>GVQLTAAQELMIQQLVAAQLQCNKRSFSDQPKVTPWPLGADPQSRDARQQRFAHFTELAIISVQEIVDFAKQVPGFLQLGREDQIALLKASTIEIMLLETARRYNHETECITFLKDFTYSKDDFHRAGLQVEFINPIFEFSRAMRRLGLDDAEYALLIAINIFSADRPNVQEPGRVEALQQPYVEALLSYTRIKRPQDQLRFPRMLMKLVSLRTLSSVHSEQVFALRLQDKKLPPLLSEIWDVHE[3x]

The liver X receptors (LXRs) alpha (LXRα, NR1H3) and beta (LXRβ, NR1H2) are members of the nuclear hormone receptor (NHR) superfamily of transcription factors that function as heterodimers with the retinoid X receptor (RXR) and activate or repress gene expression in response to binding of cholesterol derivatives or synthetic ligands. Transcriptional responses of LXRs are known to directly result from ligand-induced conformational changes in the receptor: similarly to other NHRs, in the absence of ligands or in the presence of antagonists, LXRs form complexes with corepressors, while binding of agonist ligands forces the C-terminal helix H12 of the receptor to fold into the active state that creates an activation function-2 (AF-2) coactivator-binding surface. Reaching isoform selectivity by rational structure-based drug design has proven to be difficult since the ligand-binding pockets (LBPs) of LXRα and LXRβ are virtually identical. Since the adverse lipogenic effects are considered to be largely driven by LXRα23,28, drug discovery efforts have focused on developing LXRβ-selective compounds.

In this study, we compared AZ876 with structurally related compounds AZ1–6. These compounds have a central cyclic sulfone amide scaffold with lipophilic substituents on both sides identical to AZ876, except for the tert-butyl substituent replaced by a propyl group in AZ1–3 and AZ6. The third substituent from the core is a larger elongated amine linker that is different in AZ1–6. The amine linker is mostly lipophilic with a polar group at the far end. The compounds AZ1, AZ3, and BMS-852927 have the highest affinities of 2, 4, and 3 nM, and the compounds AZ6, AZ7, and 24,25EC have the lowest affinities of 161, 105, and 133 nM, respectively. Analysis of crystal structures of LXRβ LBD in complex with WAY-254011, AZ3, AZ6, and AZ8, as well as of previously published crystal structures of LXRβ31,40,55 reveals that GW3965 and BMS-852927 are the only compounds not forming a direct hydrogen bond with LXRβ His435 and therefore they do not stabilize the His435–Trp457 activation switch crucial for the agonistic conformation of H12. Other agonists form shorter hydrogen bonds of 2.5–3.1 Å essential for proper position of H12, which correlates with their activities both in LXRβ HDX-MS and functional assays. Overall, most of the selected compounds displayed similar differential HDX patterns with a strong protection from deuterium exchange observed for the peptides lining the LBP: central part of H3, H5, β-sheet, and helices H6, H7, and H10/11.>[2x]MTTPSMEMYIEQIYMLIEEKGYARVSDIAEALAVHPSSVTKMVQKLDKDEYLIYEKYRGLVLTSKGKKIGKRLVYRHELLEQFLRIIGVD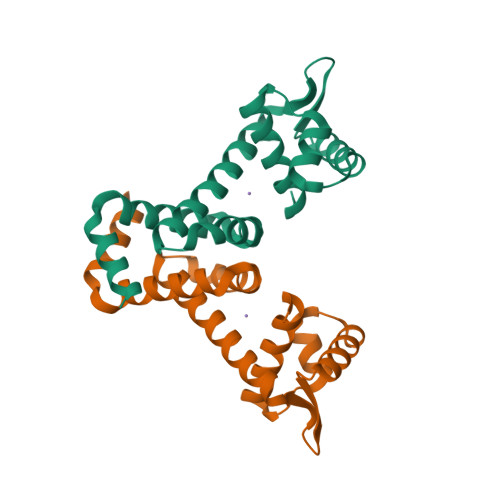EEKIYNDVEGIEHHLSWNSIDRIGDLVQYFEEDDARKKDLKSIQKKTEHHNQ4-(1,3-BENZODIOXOL-5-YLOXY)-2-[4-(1H-IMIDAZOL-1-YL)PHENOXY]-6-METHYLPYRIMIDINE 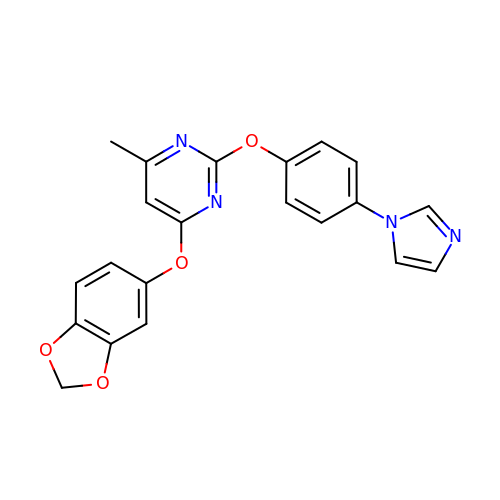| C21 H16 N4 O4 | QQBNDYARFVOEGW-UHFFFAOYSA-N>MKHHHHHHSSGENLYFQGAKKLGYKFLESLLQKDPSEVVITLATSLGLKELLSHSSMKSNFLELICQVLRKACSSKMDRQSVLHVLGILKNSKFLKVCLPAYVVGMITEPIPDIRNQYPEHISNIISLLQDLVSVFPASSVQETSMLVSLLPTSLNALRASGVD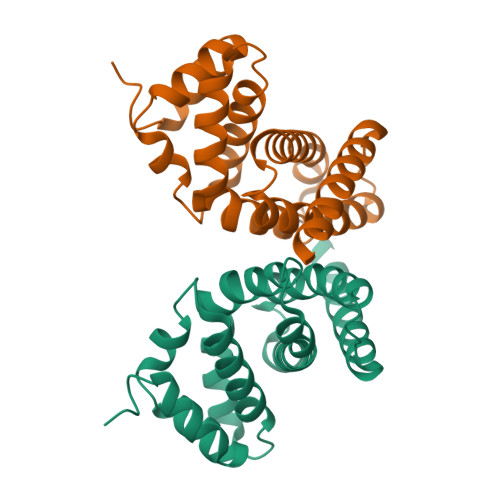IEEETEKNLEKVQTIIEHLQEKRREGTLRVDTYTL[2x]> GSHMASMKKKGSVVIVGRVVLSGDTAYAQQTRGEESTQETSQTGRDTNENCGEVQVLSTATQSFLGTAVNGVMWSVYHGAGGKTISGPKGPVNQMYTNVDQDLVGWPAPPGVKSLTPCTCGASDLYLVTRHADVVPVRRRGDTRGALLSPRPISTLKGSSGGPLLCPMGHVAGLFRAAVCTRGVAKAVDFVPVESLETTMR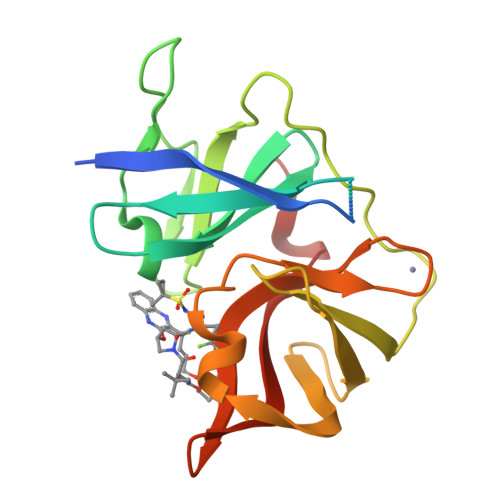SP> GSRSGVAVADESLTAFNDLKLGKKYKFILFGLNDAKTEIVVKETSTDPSYDAFLEKLPENDCLYAIYDFEYEINGNEGKESKIVFFTWSPDTAPVRSKMVYASSKDALRRALNGVSTDVQGTDFSEVSYDSVLER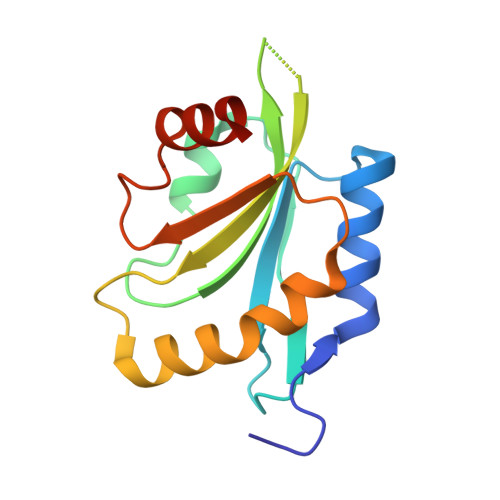VSRGAGSH>[2x]SAVLRAREVL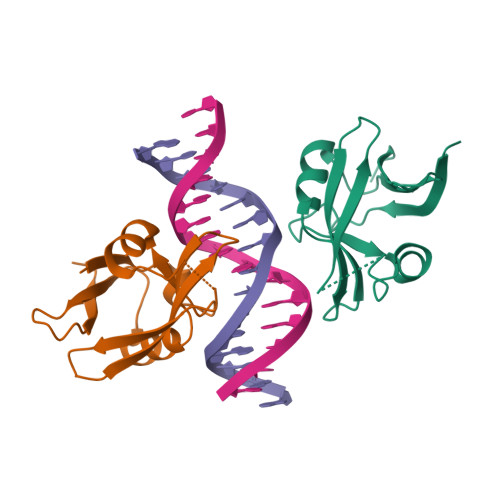FEKTVTPSDVGKLNRLVIPKQHAEKHFPLPAMTTAMGMNPSPTKGVLINLEDRTGKVWRFRYSYWNSSQSYVLTKGWSRFVKEKNLRAGDVVCFERSTGPDRQLYIHWKVRSSPV> PEVGELIEKVRKAHQETFPALCQLGKYTTNNSSEQRVSLDIDLWDKFSELSTKCIIKTVEFAKQLPGFTTLTIADQITLLKAACLDILILRICTRYTPEQDTMTFSDGLTLNRTQMHNAGFGPLTDLVFAFANQLL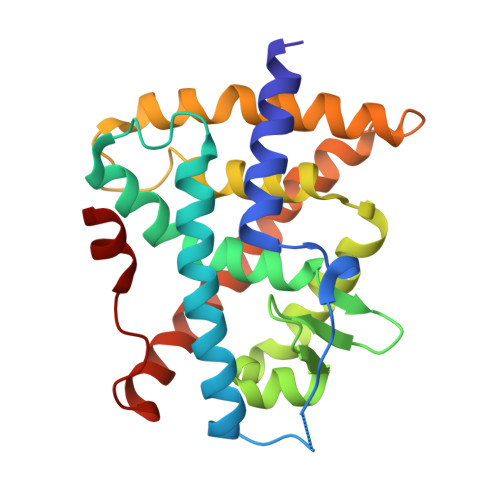PLEMDDAETGLLSAICLICGDRQDLEQPDRVDMLQEPLLEALKVYVRKRRPSRPHMFPKMLMKITDLRSISAKGAERVITLKMEIPGSMPPLIQEMLEN>[3x]GPGDKELIDWLRLQGA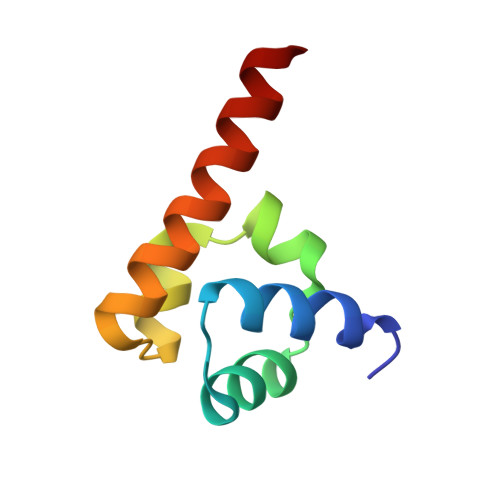DAKTIEKIVEEGYTLSDILNEITKEDLRYLRLRGGLLCRLWSAVSQYRRAQEASE> DVP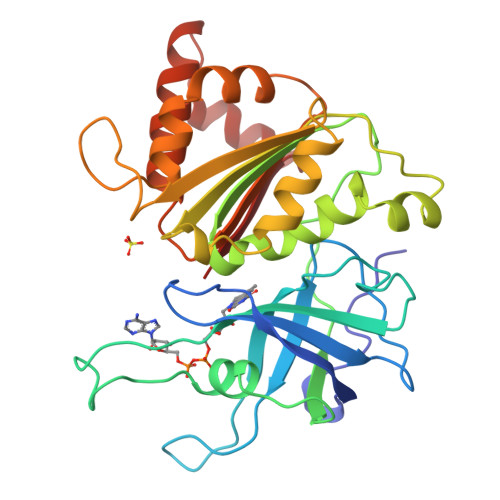VNLYRPNAPFIGKVISNEPLVKEGGIGIVQHIKFDLTGGNLKYIEGQSIGIIPPGVDKNGKPEKDRDYSIASTRHGDDVDDKTISLCVRQLEYKHPESGETVYGVCSTYLTHIEPGSEVKITGPVGKEMLLPDDPEANVIMLATGTGIAPMRTYLWRMFKDAERAANPEYQFKGFSWLVFGVPTTPNILYKEELEEIQQKYPDNFRLTYAISREQKNPQGGRMYIQDRVAEHADQLWQLIKNQKTHTYICGLRGMEEGIDAALSAAAAKEGVTWSDYQKDLKKAGRWHVETY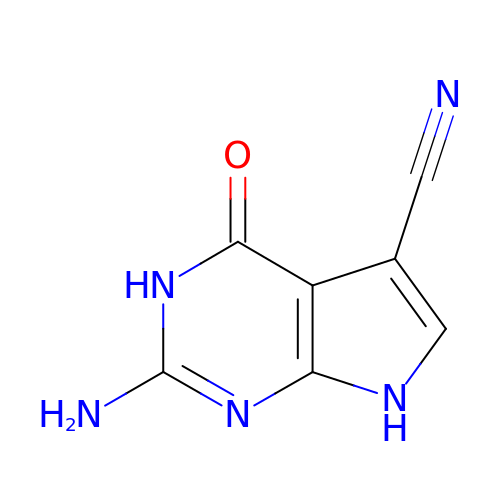2-AMINO-4-OXO-4,7-DIHYDRO-3H-PYRROLO[2,3-D]PYRIMIDINE-5-CARBONITRILE | C7 H5 N5 O | FMKSMYDYKXQYRV-UHFFFAOYSA-N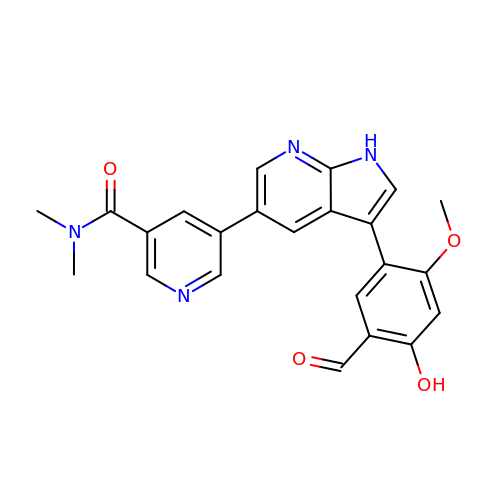5-[3-(5-methanoyl-2-methoxy-4-oxidanyl-phenyl)-1~{H}-pyrrolo[2,3-b]pyridin-5-yl]-~{N},~{N}-dimethyl-pyridine-3-carboxamide | C23 H20 N4 O4 | JYBKYHQDAOGLCV-UHFFFAOYSA-N> MQKYRLYEKDGSPVQDFNRFVKGWLDIEFGLKEHQPPKVFDTIRDKYNEAIEAVVLSGVAPRTAHKAALSTLTELLFGHDLAKELSARLDIQ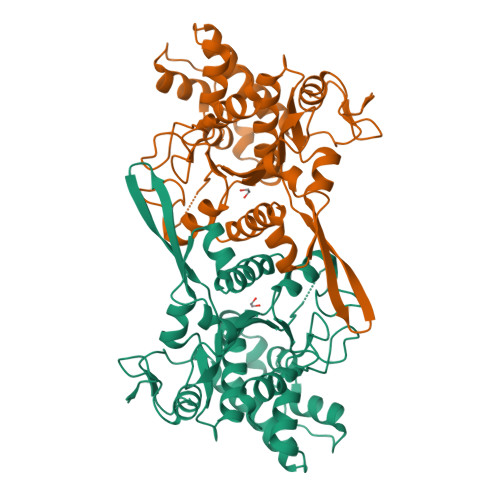PIGVGGFRSAHSQAFAKNVGENFVNLMVYALACILKDNDDVLVDKGLPPHLKKALTLSRECRIKDTLREIKIPIEGDLCVFSRSNHCNAIVISAKTRLKEVFHIGTMWALFSDVAKDEYCLNKWGLKVESSESLKDTMYVFATADMINKDGARSQGCDVERETPRNLIAMDASFFDYVFVSKMGIGHVSSDLSLKYGRESLFHELGCIIDMIEQKFDILL> MAHHHHHHMSRLMPHYSKGKTAFLCVDLQEAFSKRIENFANCVFVANRLARLHEVVPENTKYIVTEHYPK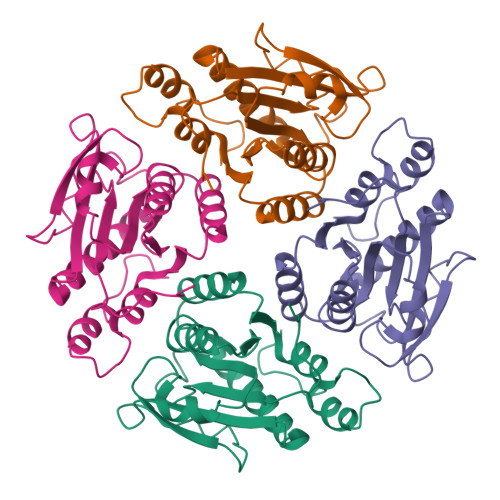GLGRIVPEITLPKTAHLIEKTRFSCVVPQVEELLEDVDNAVVFGIEGHACILQTVADLLDMNKRVFLPKDGLGSQKKTDFKAAIKLMSSWGPNCEITTSESILLQMTKDAMDPNFKRISKLLKEEPPIPL> GSHMSQPRPLLSPPETEEQLLAQAQQLSGYTLGELAALVGLVTPENLKRDKGWIGVLLEIWLGASAGSKPEQDFAALGVELKTIPVDSLGRPLETTFVCVAP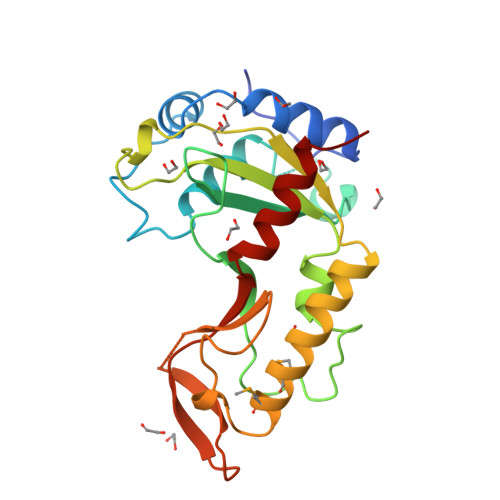LTGNSGVTWETSHVRHKLKRVLWIPVEGEASIPLAQRRVGSPLLWSPNEEEDRQLREDWEELMDMIVLGQVERITARHGEYLQIRPKAANAKALTEAIGARGERILTLPRGFYLKKNFTSALLARHFLIQ> GPMGNGMNKILPGLYIGNFKDARDAEQLSKNKVTHILSVHDSARPMLEGVKYLCIPAADSPSQNLTRHFKESIKFIHECRLRGESCLVHSLAGVNRSVTLVIAYIMTVTDFGWEDALHTVRAGRSCANPNVGFQRQLQEFEKHEVHQYRQWLKEEYG

DUSP22 is a small phosphatase containing 184 residues, and the sequence contains a catalytic domain as well as an N-terminal myristoylation site. This enzyme is broadly expressed in different tissues and plays important roles in the regulation of signaling pathways, such as inactivating the T cell receptor (TCR) signaling pathway, activating the JNK signaling pathway, and regulating the phosphorylation of focal adhesion kinase (FAK). The phosphatase domain of DUSP22 consists of five twisted β-sheets and six α-helices, and the structural scaffold is similar to that of DUSP3 (VHR), while DUSP22 does not contain an N-terminal α-helix surrounded by the N-loop. In this region, the catalytic activity is facilitated by C88 in the P-loop and D57 in the D-loop, and the hydrogen bonding network is formed by D57 in the D-loop, S93 in the P-loop, and N128 in the N-loop.

The S93 mutants were combined with a second mutation, C88S, to produce proteins for growing better crystals, which improved the resolution (<1.6 Å) and helped to determine the structures. In contrast, the N93 in the crystal structure of C88S/S93N had a different effect and formed the hydrogen bonding with the side chain of D57 and the backbone amide of N128. The side chain of N128 also interacted with the side chain of D57. The DPN–triloop interaction formed but was not precise. This DPN–triloop interaction lacked a hydrogen bond between the side chains of N93 and N128, and the positions of D57 and N128 were shifted due to a spatial barrier from N93. The decrease in catalytic efficiency in S93N was associated with this conformational change. This result indicated that the formation of the DPN–triloop interaction through S93 induced precise spatial localization to stabilize active site structure and maintain phosphatase activity. Even though S93N interacts with N128 and D57 in the crystal structure, the positions of D57 and N128 are different from those in the WT, and the N-loop and the D-loop are shifted. In the S93N mutant, N93 is a barrier that blocks D57 close to the substrate and decreases kcat.>MAMPLDWDKLRIFHAAAEAGSFTHAADKLHLSQSAISRQVSALEQDVGVKLFHRHARGLILTEQGELLYRTAHDVLLKLETVKMQLTETTEKPSGKLRVTTTVGLGQGWLTDKVQEFLQLYPEMSIQLILDNEELDVNMRHADCAIRLRQPQQSDLIQRKLFTVHMHVYAAPSYINRHGEPQSVEDLDNHRIISFGEPAPNYLLDVNWLENAGRSSDNTRIPHLQINSQTSIKRACLLGIGIACLPDYIVGRDPGLIQLSLAADIPSFDTYFCYPDEMKNAAKLKAFRDFIVAKARN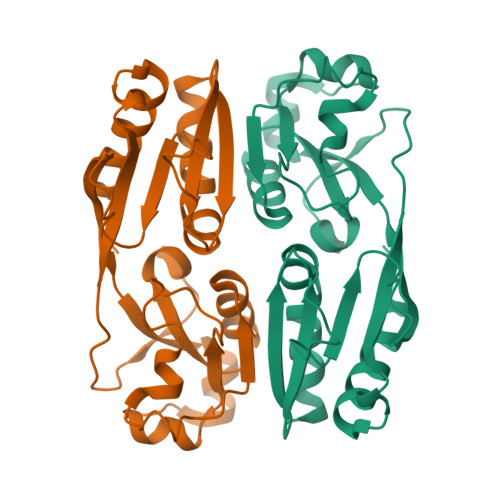WNFGTSAWSHPQFEK[2x]>DYFQGAMGSKPAYSFHVTADGQMQPVPFPPDALIGPGIPRHARQINTLNHGEVVCAVTISNPTRHVYTGGKGCVKVWDISHPGNKSPVSQLDCLNRDNYIRSCKLLPDGCTLIVGGEASTLSIWDLAAPTPRIKAELTSSAPACYALAISPDSKVCFSCCSDGNIAVWDLHNQTLVRQFQGHTDGASCIDISNDGTKLWTGGLDNTVRSWDLREGRQLQQHDFTSQIFSLGYCPTGEWLAVGMESSNVEVLHVNKPDKYQLHLHESCVLSLKFAYCGKWFVSTGKDNLLNAWRTPYGASIFQSKESSSVLSCDISVDDKYIVTGSGDKKATVYEVIY[2x]

Transducin‐like enhancer (TLE) proteins are transcriptional co‐repressors that modulate key pathways for developmental and oncogenic signalling, such as the Notch and Wnt pathways. The TLE proteins do not bind directly to DNA to exert their repressive effect on gene transcription; instead, they utilise their WDR domains to bind to DNA‐bound transcription factors. Given that TLE1 does not bind to DNA directly, and that its repressive and potentially oncogenic role relies on the ability of the WDR domain to bind to transcription factors, blocking of this interaction has been suggested as a possible treatment for cancers with elevated TLE1 activity. Herein, the structure‐enabled design and synthesis of a constrained peptide inhibitor of TLE1 is reported.

Briefly, we grew apo crystals of the TLE1 WD40 domain by using slightly modified previously published conditions and succeeded in solving the structure of cyclic peptide 18 bound to TLE1 to 2.18 Å resolution by soaking with a 2.5 mm solution of 18. The asymmetric unit contained two TLE1 monomers and the electron density was evident in both binding sites. Chain A showed strong ligand density and allowed us to model cyclic peptide 18 with full occupancy. The ligand density in chain B was weaker and refined at a lower occupancy (0.83). Overall, the binding mode of the constrained peptide is almost identical to that of the published acyclic peptide‐bound structure. The overall root‐mean‐square deviation (RMSD) between the two structures is 0.55 Å. The N‐terminal phenylalanine side chain of the constrained peptide occupies a similar position to that of the methionine side chain, with the aromatic side chain efficiently packing against the hydrophobic part of Glu 550; this potentially explains the slightly higher affinity of acyclic FWRPW, compared with that of the MWRPW peptide. The most significant difference between the cyclic peptide conformation and the bound SMRWPW conformation is the linker, which appears to cause a slight change in position of the N‐terminal tryptophan and could go some way to explain the lower affinity of 18 compared with that of the linear FWRPW peptide. The crystal structure of the constrained peptide bound to TLE1 suggests that the linker causes some strain in the molecule that may, at least partially, explain the lower affinity.~{N}-[4-[5-[(dimethylamino)methyl]-1-methyl-pyrazol-3-yl]pyrimidin-2-yl]-3-methyl-1-(5-methyl-1,3,4-oxadiazol-2-yl)imidazo[1,5-a]pyridin-7-amine | C22 H24 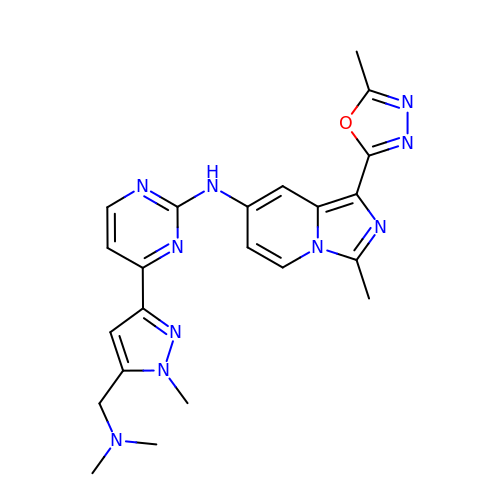N10 O | PAZNLQHSWVMGIW-UHFFFAOYSA-N> GGACGGAGGCGCGCCCGAGAUGAGUAGGCUGUCCCAUCAGGGGAGGAAUCGGGGACGGCUGAAAGGCGAGGGCGCCGAAGCGAGCAGAGUUCCUCC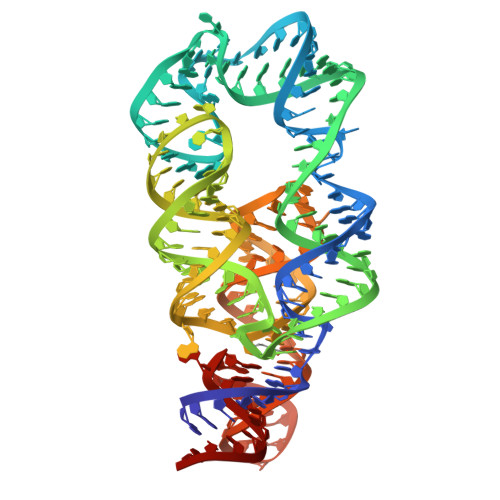CGCUCUGCUUGGCUGGGGGUGAGGGGAAUACCCUUACCACUGUCGCGAAAGCGGAGAGCCGUCCA>GAMASSSHSRAGQSAAGAAPGGGVDTRDAEMPATEKDLAEDAPWKKIQQNTFTRWCN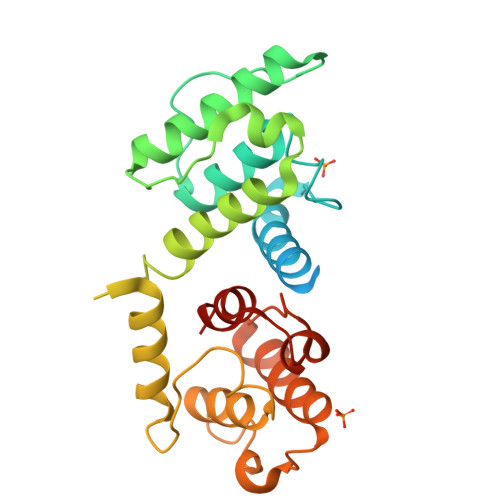EHLKCVSKRIANLQTDLSDGLRLIALLEVLSQKKMHRKHNQRPTFRQMQLENVSVALEFLDRESIKLVSIDSKAIVDGNLKLILGLIWTLILHYSISMPMWDEEEDEEAKKQTPKQRLLGWIQNKLPQLPITNFSRDWQSGRALGALVDSCAPGLCPDWDSWDASKPVTNAREAMQQADDWLGIPQVITPEEIVDPNVDEHSVMTYLSQFPKAKL[2x]> MEP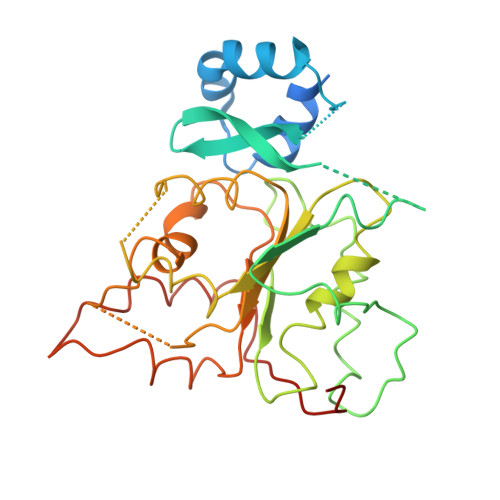IGRSLQGVTGRPDFQKRLEQMKEKVMKDQDVQAFLKENEEVIDQKMIEKSLNKLYEYIEQSKNCSYCSEDENCNNLLEGYHPKLVVNGRSIDIEYYECPVKRKLDQQKKQQSLMKSMYIQQDLLGATFQQVDISDPSRLAMFQHVTDFLKSYNETGKGKGLYLYGKFGVGKTFMLAAIANELAEKEYSSMIVYVPEFVRELKNSLQDQTLEEKLNMVKTTPVLMLDDIGAESMTSWVRDEVIGTVLQHRMSQQLPTFFSSNFSPDELKHHFTYSQRGEKEEVKAARLMERILYLAAPIRLDGENRRHPHHHHHH> MADEERLKEFKEANKIVFDPNTRQVWENQNRDGTKPATTFQSEEDIKRA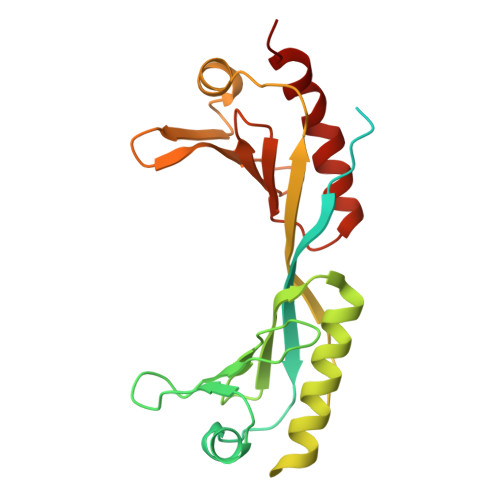APESEKDTSATSGIVPTLQNIVATVTLGCRLDLKTVALHARNAEYNPKRFAAVIMRIREPKTTALIFASGKMVVTGAKSEDDSKLASRKYARIIQKIGFAAKFTDFKIQNIVGSCDVKFPIRLEGLAFSHGTFSSYEPELFPGLIYRMVKPKIVLLIFVSGKIVLTGAKQREEIYQAFEAIYPVLSEFRKM(4-VINYLPHENYL)METHANESULFONIC ACID | C9 H10 O3 S | 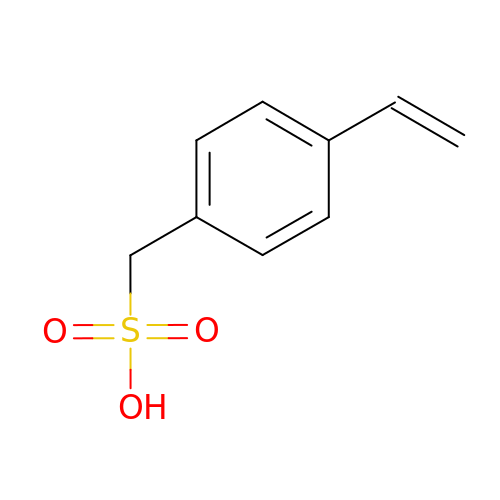SDXKWPVFZWZYNK-UHFFFAOYSA-N>MKILLTGFEPFGGDDKNPTMDIVEALSERIPEVVGEILPVSFKRAREKLLKVLDDVRPDITINLGLAPGRTHISVERVAVNMIDARI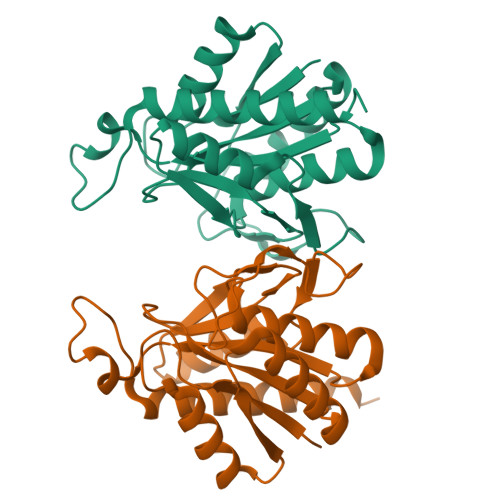PDNDGEQPKDEPIVEGGPAAYFATIPTREIVEEMKKNGIPAVLSYTAGTYLCNFAMYLTLHTSATKGYPKIAGFIHVPYTPDQVLEKKNTPSMSLDLEIKGVEIAIRVAQSALHSSQLR[2x]> PNVKRGNFTEQEEDLIIRLHKLLGNRWSLIAKRVPGRTDNQVKNYWNTHLSK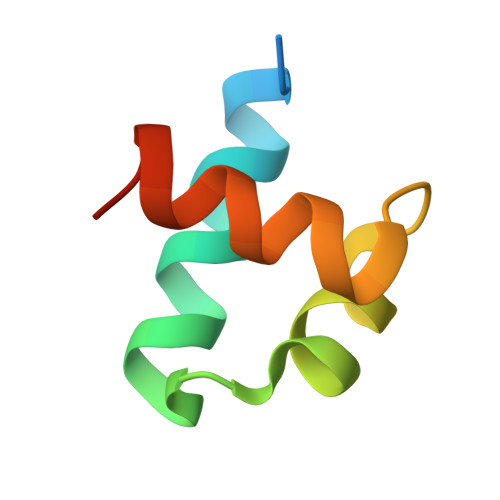KL> MIVSDIEANALLESVTKFHCGVIYDYSTAEYVSYRPSDFGAYLDALEAEVARGGLIVFHNGHKYDVPALTKLAKLQLNREFHLPRENCIDTLVLSRLIHSNLKDTDMGLLRSGKLPGALEAWGYRL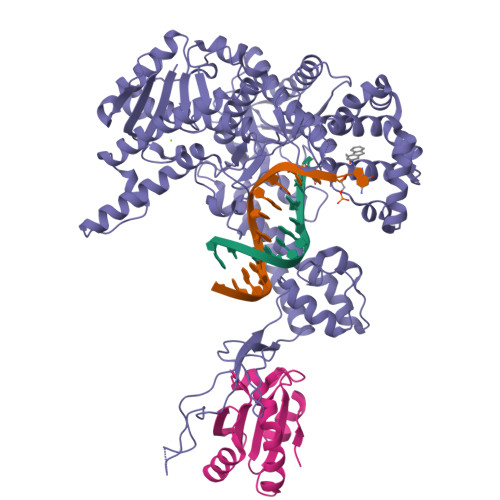GEMKGEYKDDFKRMLEEQGEEYVDGMEWWNFNEEMMDYNVQDVVVTKALLEKLLSDKHYFPPEIDFTDVGYTTFWSESLEAVDIEHRAAWLLAKQERNGFPFDTKAIEELYVELAARRSELLRKLTETFGSWYQPKGGTEMFCHPRTGKPLPKYPRIKTPKVGGIFKKPKNKAQREGREPCELDTREYVAGAPYTPVEHVVFNPSSRDHIQKKLQEAGWVPTKYTDKGAPVVDDEVLEGVRVDDPEKQAAIDLIKEYLMIQKRIGQSAEGDKAWLRYVAEDGKIHGSVNPNGAVTGRATHAFPNLAQIPGVRSPYGEQCRAAFGAEHHLDGITGKPWVQAGIDASGLELRCLAHFMARFDNGEYAHEILNGDIHTKNQIAAELPTRDNAKTFIYGFLYGAGDEKIGQIVGAGKERGKELKKKFLENTPAIAALRESIQQTLVESSQWVAGEQQVKWKRRWIKGLDGRKVHVRSPHAALNTLLQSAGALICKLWIIKTEEMLVEKGLKHGWDGDFAYMAWVHDEIQVGCRTEEIAQVVIETAQEAMRWVGDHWNFRCLLDTEGKMGPNWAICH;> SDKIIHLTDDSFDTDVLKADGAILVDFWAEWCGPCKMIAPILDEIADEYQGKLTVAKLNIDQNPGTAPKYGIRGIPTLLLFKNGEVAATKVGALSKGQLKEFLDANLA> GAMDPSSPNYDKWEMERTDITMKHKLGGGQYGEVYEGVWKKYSLTVAVKTLKEDTMEVEEFLKEAAVMKEIKHPNLVQLLGVCTREPPFYIITEFMTYGNLLDYLRECNRQEVSAVVLLYMATQISSAMEYLEKKNFIHRDLAARNCLVGENHLVKVADFGLSRLMTGDTYTAHAGAKFPIKWTAPESLAYNKFSIKSDVWAFGVLLWEIATYGMSPYPGIDLSQVYELLEKDYRMERPEGCPEKVYELMRACWQWNPSDRPSFAEIHQ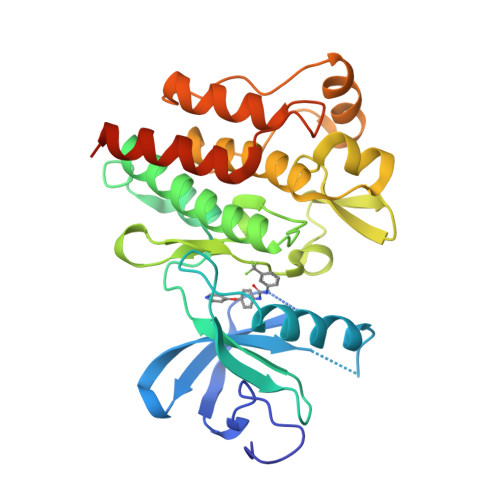AFETMFQESSISDEVEKELGKRGT> MALKDDAVLIAARGYVYTAAVGTAAPTPSQLKLIDLEHPEAWDRTGWDLVGHTSEDDLPEF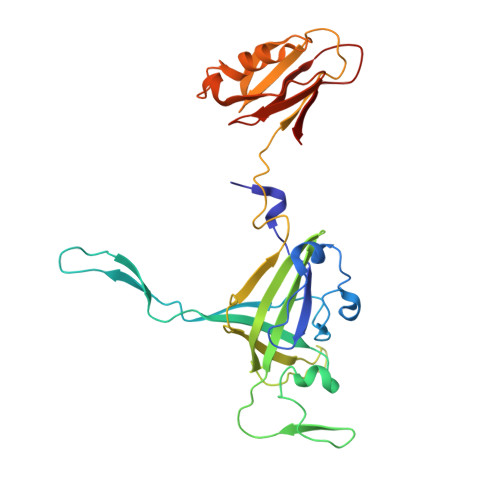GFDGGDSEVRGSWQKKKLREVETEEIADYVVINLTQFDETALELYFGPNQSATPGIFGVKSGSVVNERALLIVIVDNDVRLGFHARKASLKREDAISLATDEFGALPVRATFLDYQSYNLYEWIEEDWFNAVDAPVVYLLDLGGATGGDYTLLVGGKSTGDIAYNANASAIKTAIGAVDDGVAESAWTVTADGSDFEISGPLAVALGVDSTTGGSGVTVDVV>GMSINSREVLAEKVKNAVNNQPVTDMHTHLFSPNFGEILLWDIDELLTYHYLVAEVMRWTDVSIEAFWAMSKREQADLIWEELFIKRSPVSEACRGVLTCLQGLGLDPAT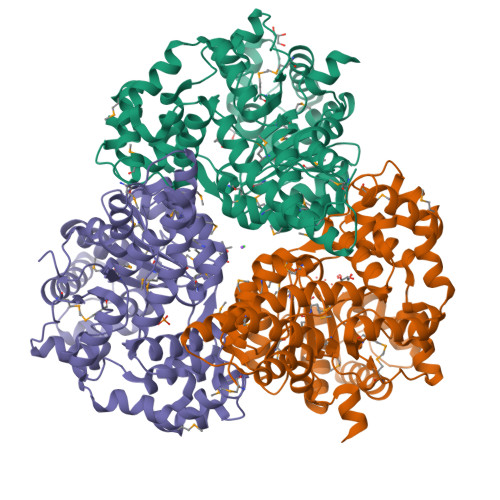RDLQVYREYFAKKTSEEQVDTVLQLANVSDVVMTNDPFDDNERISWLEGKQPDSRFHAALRLDPLLNEYEQTKHRLRDWGYKVNDEWNEGSIQEVKRFLTDWIERMDPVYMAVSLPPTFSFPEESNRGRIIRDCLLPVAEKHNIPFAMMIGVKKRVHPALGDAGDFVGKASMDGVEHLLREYPNNKFLVTMLSRENQHELVVLARKFSNLMIFGCWWFMNNPEIINEMTRMRMEMLGTSFIPQHSDARVLEQLIYKWHHSKSIIAEVLIDKYDDILQAGWEVTEEEIKRDVADLFSRNFWRFVGRNDHVTSVKVEQQT[12x]>MSEAAHVLITGAAGQIGYILSHWIASGELYGDRQVYLHLLDIPPAMNRLTALTMELEDCAFPHLAGFVATTDPKAAFKDIDCAFLVASMPLKPGQVRADLISSNSVIFKNTGEYLSKWAKPSVKVLVIGNPDNTNCEIAMLHAKNLKPENFSSLSMLDQNRAYYEVASKLGVDVKDVHD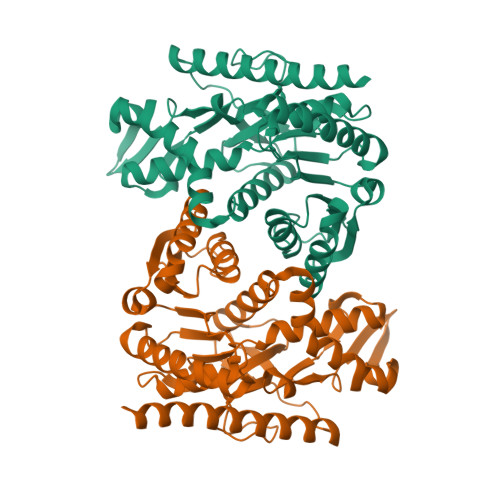IIVWGNHGESMVADLTQATFTKEGKTQKVVDVLDHDYVFDTFFKKIGHRAWDILEHRGFTSAASPTKAAIQHMKAWLFGTAPGEVLSMGIPVPEGNPYGIKPGVVFSFPCNVDKEGKIHVVEGFKVNDWLREKLDFTEKDLFHEKEIALNHLAQLEHHHHHH[2x]>[2x]MLLNLDVRMQLKELAQKEFK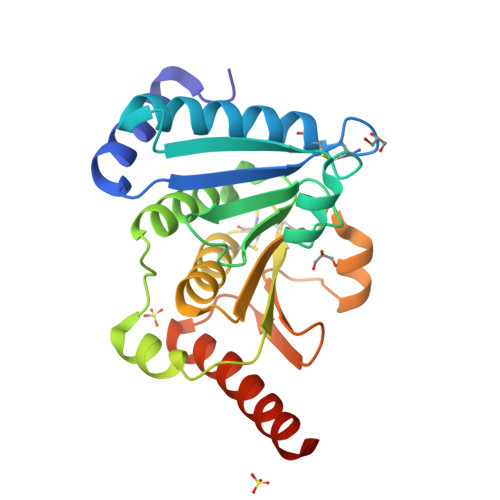EPVSIKLFSQAIGCESCQTAEELLKETVEVIGEAVGQDKIKLDIYSPFTHKEETEKYGVDRVPTIVIEGDKDYGIRYIGLPAGLEFTTLINGIFHVSQRKPQLSEKTLELLQVVDIPIEIWVFVTTSCGYCPSAAVMAWDFALANDYITSKVIDASENQDLAEQFQVVGVPKIVINKGVAEFVGAQPENAFLGYIMAVYEKLKREKEQALEHHHHHH>AQTVPYGIPLIKADKVQAQGFKGANVKVAVLDTGIQASHPDLNVVGGASFVAGEAY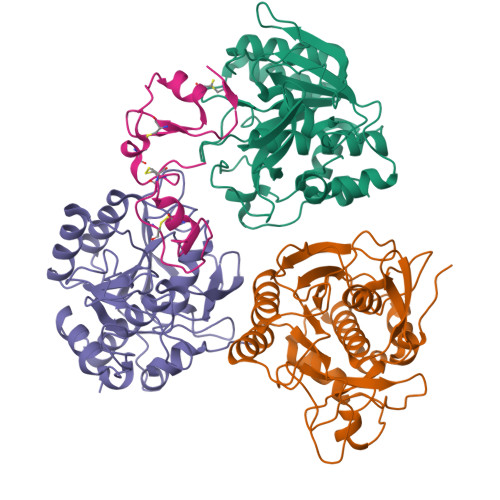NTDGNGHGTHVAGTVAALDNTTGVLGVAPSVSLYAVKVLNSSGSGSYSGIVSGIEWATTNGMDVINMSLGGASGSTAMKQAVDNAYARGVVVVAAAGNSGSSGNTNTIGYPAKYDSVIAVGAVDSNSNRASFSSVGAELEVMAPGAGVYSTYPTNTYATLNGTSMASPHVAGAAALILSKHPNLSASQVRNRLSSTATYLGSSFYYGKGLINVEAAAQ[3x];> APCPHTYKPVCGANGEVYDNECFLNKAGIEPAESWETCRGHELCPSVCTEEYDPVCVEGKIYGNRCMQSHFCGKV> GSHMKIKACIDEVTTTLEETKFLTNKLLLFADINGKLYHDSQNMLRGEDMSFLEKDAPYMVGDVITSGDITCVVIPSKKAGGTTEMLSRALKKV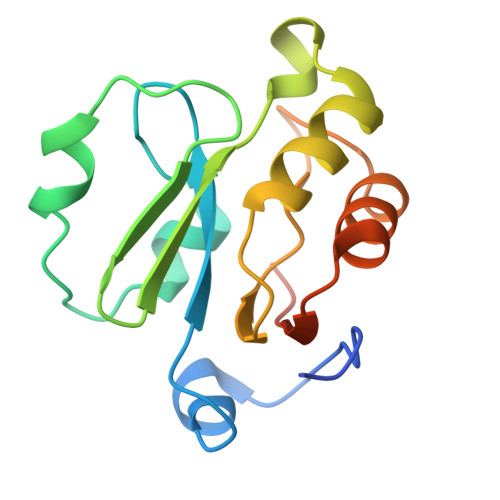PVDEYITTYPGQGCAGYTLEEAKTALKKCKSAFYVLPSEAPNAKEEIL>[5x]MTITYTSQVANARLGSFSRLLLCWRGSIYKLLYGEFLIFLLCYYIIRFIYRLALTEEQQLMFEKLTLYCDSYIQLIPISFVLGFYVTLVVTRWWNQYENLPWPDRLMSLVSGFVEGKDEQGRLLRRTLIRYANLGNVLILRSVSTAVYKRFPSAQHLVQAGFMTPAEHKQLEKLSLPHNMFWVPWVWFANLSMKAWLGGRIRDPILLQSLLNEMNTLRTQCGHLYAYDWISIPLVYTQVVTVAVYSFFLTCLVGRQFLNPAKAYPGHELDLVVPVFTFLQFFFYVGWLKVAEQLINPFGEDDDDFETNWIVDRNLQVSLLAVDEMHQDLPRMEPDMYWNKPEPQPPYTAASAQFRRASFMGSTFNISLNKEEMEFQPNQEDEEDAHAGIIGRFLGLQSHDHHPPRANSRTKLLWPKRESLLHEGLPKNHKAAKQNVRGQEDNKAWKLKAVDAF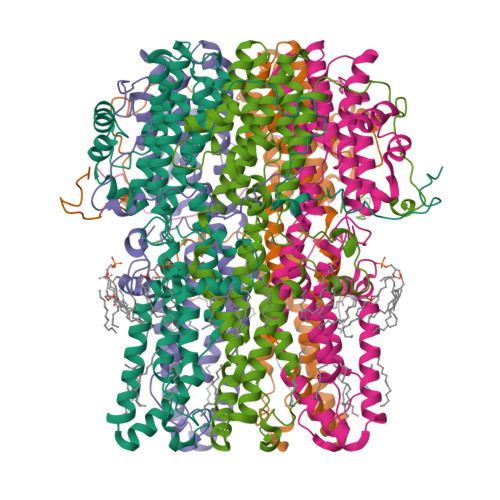KSAPLYQRPGYYSAPQTPLSPTPMFFPLEPSAPSKLHSVTGIDTKDKSLKTVSSGAKKSFELLSESDGALMEHPEVSQVRRKTVEFNLTDMPEIPENHLKEPLEQSPTNIHTTLKDHMDPYWALENRDEAHS>[2x]MKHSLPDLPYDYGALEPHINAQIMQLHHSKHHAAYVNNLNVTEEKYQEALAKGDVTAQIALQPALKFNGGGHINHSIFWTNLSPNGGGEPKGELLEAIKRDFGSFDKFKEKLTAASVGVQGSGWGWLGFNKERGHLQIAACPNQDPLQGTTGLIPLLGIDVWEHAYYLQYKNVRPDYLKAIWNVINWENVTERYMACKK

Human manganese superoxide dismutase (MnSOD) is a CPET-based oxidoreductase found in the mitochondrial matrix that reduces ROS levels by eliminating O2•− with the unpaired electrons of the active site metal. The Mn ion is coordinated to inner-sphere residues His26, His74, His163, Asp159, and a single-oxygen species that could be either H2O or –OH (designated WAT1). Trivalent Mn oxidizes O2•− to O2 (k1 = 1.5 nM−1 s−1)8 and the resulting divalent Mn reduces another O2•− molecule to H2O2 (k2 = 1.1 nM−1 s−1). The second sphere of MnSOD harbors five residues (His30, Tyr34, Gln143, Glu162, and Tyr166) and information about their protonation states would be of significant value in deciphering a catalytic mechanism.

To visualize the effect of the electronic state of the metal on the active site protons, all-atom, D-labeled neutron structures were obtained for Mn3+SOD and Mn2+SOD to resolutions of 2.20 and 2.30 Å, respectively. The two data sets collected were from the same crystal treated with appropriate oxidizing and reducing chemicals and the redox conditions were maintained during each data collection. For the reduced resting state described by chain B of Mn2+SOD, Tyr166 and His30 now share the proton originating from Nε2(His30) with a LBHB, His30 is protonated on Nδ1, and Tyr34 is no longer ionized. Gln143 and WAT1 have undergone a proton transfer where WAT1 is now H2O and Gln143 is an amide anion. Gln143 forms SSHBs with WAT1 and Trp123 presumably to stabilize its ionized form. An SSHB of 1.5 Å is seen between the Oε1 of Gln143 and Dε1 of Trp123 in the reduced state. Serendipitously, one of the active sites of the Mn2+SOD neutron structure has density for an unexpected sixth-coordinate –OD ligand (designated OL for anionic oxygen ligand), and the Mn–Oδ2(Asp159) bond is stretched from 1.95 to 2.44 Å. The third active site state is a six-coordinate Mn2+ with –OH-bound opposite Asp159 described by chain A of Mn2+SOD. Tyr166 and His30 share a LBHB and His30 is Nδ1 protonated, like the reduced resting state, while Tyr34 is ionized like the oxidized resting state. Gln143 in the amide form but forms an SSHB with −OH(WAT1) and also Trp123.>MTSDKFLSGVVEGFYGKPWSFEQ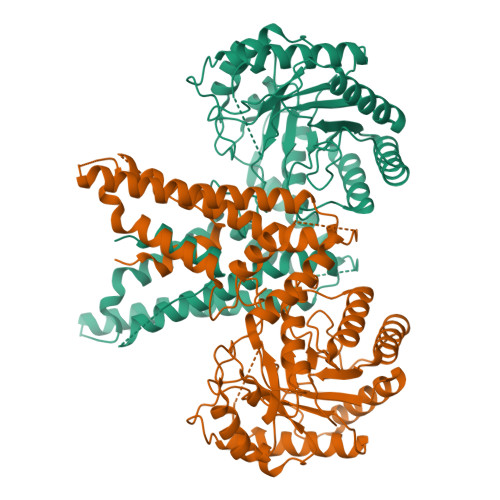RKTLFSNMAKWGLNTYMYGPKDDEKHRAAWKQAYSKREGDSLRALIRAAEESGILFIYAISPGVDITYSSNRDMKFLKDKLDQIRNFGCNSFAIFFDDIDTVMCLQDQEEFESFAAAQVEVTNEIYKYLGMPANFLFCPTEYCAARADPNVKESKYLVTVGTGLHSDIHIMWTGPKVVSNKISVESILELQTVLRRKPVIWDNIHANDYEQGRLNLGPYDCRPAELMESLNGIFTNPNCEFELNYVPIRTFSLWCQSKRTRFNYDVEKALEQSIREWTEEFCIPRLPDGYLLEADTSDTNVNEYMDDEMQSDSRPISPANSMETDKDELTVKDIRLLVELFYLPQKHGKTANDLLAQAKWLKSNFRIAALSRKPNDTSEGSNLDEHNTDYIAAKEWDKRFSKFRSICQIIHQFGDRLMTCRNRVLLYEVYNYVADLCGILYHLISRIHSLANPEKLEKRSDSEQSSFRYGGFVGDIHRLIVSTDEYEESTLKNSDAYVIRPFMPSDEETLYDLCLKSCIENSNGDEIYKREPRIIGDRDLGAYIYLHPEYIYVLEDDRDKICGYLCGALDSKQFYERYESEWLTQIRDRHPQPENDIASWTPEEIVANSFYNFTPPTDVSVLYLSHLEARFDSSVPEKVIKRIIRFILEQLKAKGSYGASMLIDSWRTNLRRIFTSMGFVDLQEYSWMSEQKCMIAIKLM[2x]>[2x]MQTRSSRMAGFGHAVPARCVDNAEIEASLGLEAGWIERRTGIRSRYWAEAGDTLSGLAERAGRMALEDAKINADDIALTLLATSTPDHLLPPSAPLLAHRLGLTRSGAIDLAGACSGFLYALTLADGFVRTYGRAVLVAAANILSRRINPAERASAVLFADAAGAVVLTPCPEVKRGVLSADLVADGSGYDLIQIAAGGSSQPFSAGMIAEDALMTMRDGREVFSRAVAL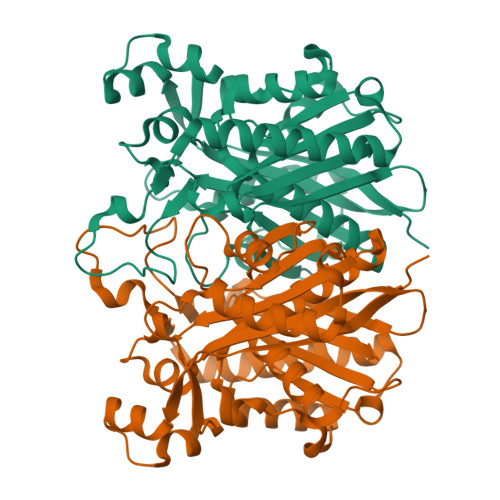MTNTSQRVLHEAELTAADISRFVPHQANARMSDAVCGNLGIEREKTVRTIGSFGNSSAATIPLSLSITNAERPLAGGETLLLTAAGAGMTGGAVVYRV>MAPIAVGDVLPDGKLAYFDEQDQLQ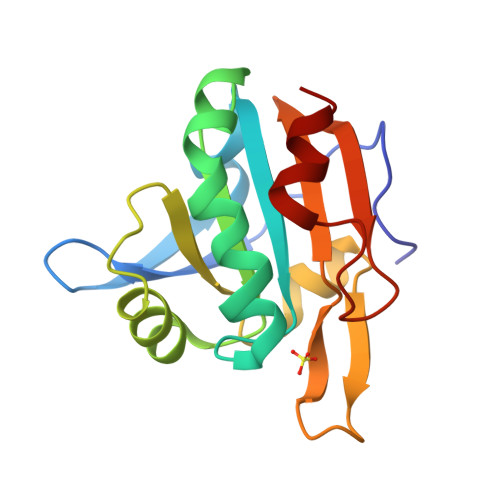EVSVHSLVAGKKVILFGVPGAFTPTCSLKHVPGFIEKAGELKSKGVTEILCISVNDPFVMKAWAKSYPENKHVKFLADGSATYTHALGLELDLQEKGLGTRSRRFALLVDDLKVKAANIEGGGEFTVSSAEDILKDL[4x]> GAACGACACCGA;> CGGGGACTC;> TCGC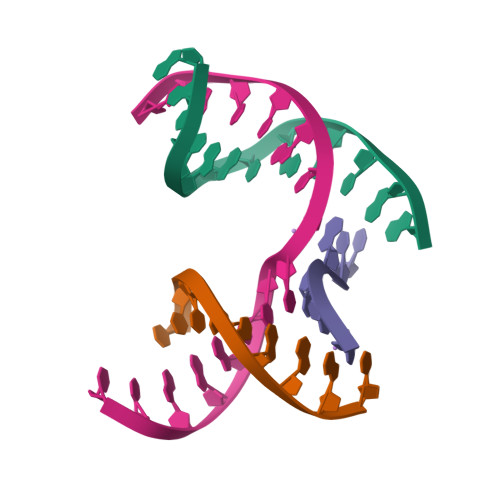CG;> TCGAGTCCGTGTCGT>MGSDKIHHHHHHENLYFQGMTFVESMQRRAVLAQKRLVLPEACEQRTLEAARLIVFRNIAAKVFLVGCERDIKNTADRCGIDLTDMVVIDPSVSKHRDQFAERYFQKRKHKGISLAQAAEDMRDPLRFAAMMLDQGHADAMVAGAENTTARVLRAGLTIIGTLPSVKTASSCFVMDTNNPRLGGTRGLFIFSDCAVIPTPTAEQLADIACSAAESCRTFIGEEPTVALLSYSTKGSGGDSDENILRVREAVRILHERRVDFTFDGELQLDAALVPKITEKKAPHSPITGKVNTLVFPDLSSGNIGYKLVQRLSDADAYGPFLQGFAKPLSDLSRGCSVEDIVAACAVTLVQSNGR[2x]

As a part of the hypothesis, we have proposed that T. pallidum contains an acetogenic energy-conservation pathway that catabolizes D-lactate, yielding acetate, reducing equivalents for the generation and maintenance of chemiosmotic potential, and ATP. To continue the validation of this pathway, thus creating a more comprehensive view of T. pallidum metabolism, we have characterized the protein TP0094 (UniProt Acc. #O83132), the putative phosphotransactetylase (Pta; EC 2.3.1.8) catalyzing the penultimate step in the acetogenic pathway, i.e., displacing the CoA moiety of acetyl-CoA with a phosphate, yielding acetyl phosphate. In the current study, we focused on another enzyme ostensibly involved in treponemal acetogenesis, phosphotransacetylase (Pta). This enzyme is putatively identified as TP0094 and, in this study, we determined a high-resolution (1.95 Å) X-ray crystal structure of the protein, finding that its fold comports with other known Pta enzymes. From these facts, we infer that TP0094 can act as a bona fide Pta enzyme in T. pallidum, and we propose to refer to it as TpPta henceforth.

There were two molecules in the asymmetric unit, and nearly all residues present in the protein construct could be modeled. The structure is divided into two domains, called “Domain I” and “Domain II” according to established nomenclature for Pta enzymes. Domain I, (amino-acids 1–141 and 309–334), which contains both the amino- and carboxyl-termini, has a central, 5-stranded parallel β-sheet that is flanked by several helical elements. Domain II (amino-acids 150–305) also features a mostly parallel central β-sheet, but the penultimate of its six strands is antiparallel. Between the two domains is a cleft that is implicated in catalysis by other Ptas. Although several water molecules are observed in this cleft, there was no evidence of substrates or products bound therein. Monomer-monomer contacts are made solely through the respective Domains I. Monomer A and Monomer B have essentially the same conformation: superposing the 324 common Cα atoms of the monomers results in a root-mean-square deviation (r.m.s.d.) of 0.5 Å. The two monomers are intimately associated, burying 2,640 Å2 of surface area, and estimates of the energetics of this dimer using PISA indicate a strong likelihood that the dimer is stable in solution (i.e. ΔGint = −22.6 kcal/mol). Moreover, the C and D monomers adopt an “intermediate” conformation in which Domain II is rotated only by about 5–7° relative to the open form. It is this intermediate conformation that most resembles the conformation displayed by both monomers of TP0094. Thus, the conformations of Pta may be important for the enzyme’s catalytic cycle, and the intermediate conformation of TP0094 comports with its lack of substrates or products in its putative active site.The completed glycoconjugate is exported by the WzmWzt ABC transporter to the periplasm where the O antigen is transferred to the lipid-A core to form a mature LPS molecule that is shuttled to the outer leaflet of the OM5. Wzm forms the ABC transporter’s membrane-embedded permease domain and Wzt contains the classical cytosolic nucleotide-binding domain (NBD). The CBD is fused in tandem to the C-terminal end of the conserved NBD of Wzt. The CBD is essential for capped O antigen export in vivo as transporters lacking the domain or carrying CBDs with compromised cap binding activities fail to export their lipid-linked substrates.

Indeed, each CBD monomer binds the methylated monosaccharide with about 234 µM affinity and at a 1:1 molar ratio. No binding is observed to unmodified D-mannose, suggesting that the CBD specifically recognizes the sugar’s O3 substitution. To delineate how the CBD recognizes the cap, we crystallized the isolated A. aeolicus CBD in the presence of 3-O-Me-D-Man and solved the molecular structure at 1.6 Å resolution by molecular replacement. The monosaccharide binds to each CBD protomer on their flat β-sheet surfaces, formed by β-strands 3, 4, 6 and 7. Specific contacts are formed between the ring oxygen and the δ2 amide from Asn313, the C2 hydroxyl and the ε2-nitrogen from His350, as well as the C4 hydroxyl and the carbonyl backbone from Ile299. The C6 hydroxyl group, which is absent in Rha, only undergoes water-mediated interactions with the carbonyl of Met353. Compared to CBD’s apo conformation, these interactions position its loop connecting β-strands 6 and 7 (residues 352-356, hereafter referred to as ‘trap-loop’) towards the ligand-binding site, thereby trapping the O antigen cap. The 3-O-methyl moiety fits into a small hydrophobic pocket formed by Leu300, Thr346, Ala348 and Trp362. The indole ring from Trp362 stacks against the methyl cap through CH-π interactions. Altogether, our data demonstrate that A. aeolicus CBD specifically recognizes the methyl-cap on the non-reducing end sugar of the O antigen via interactions that would also be consistent with 3-O-methyl-Rha forming the cap.

>GSNFKAVIKEVRLKSEHGYTNNFPSGDTLFIELDVEAKEDLQDVVAGILIRDRFGQDIFGINTYLMEKKVELKKGKYLFTFKMPLNLAPGKYTLTVALHKGMDHAQECYHWIDNVCNFEVNGFKKEQFVGVCYLPTEFNYRKIP[2x]5'-{[(3S)-3-amino-3-carboxypropyl]({1-[(3-chlorophenyl)methyl]azetidin-3-yl}methyl)amino}-5'-deoxyadenosine | C25 H33 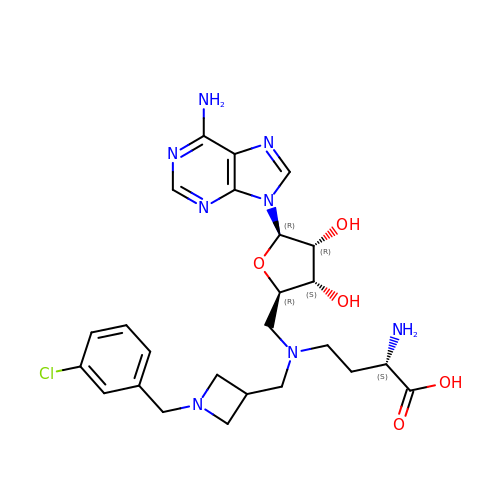Cl N8 O5 | XCVJSTZYHUNTCU-XCPBYIKRSA-N The attachment of myristate to the N-terminal glycine of certain proteins is largely a co-translational modification catalyzed by N-myristoyltransferase (NMT), and involved in protein membrane-localization. Using coenzyme A (CoA)-activated lipid, NMT transfers myristate to the substrate protein, after removal of the initiator methionine, in a predominantly co-translational process (Ritzefeld et al., 2017, Schlott et al., 2018). Pathogen NMT is a validated therapeutic target in numerous infectious diseases including malaria. PvNMT possesses 80% sequence identity and 93% similarity to PfNMT and is an excellent platform for structural studies, while to date PfNMT has proven intractable for X-ray crystallography.

IMP-1002 is a previously undisclosed member of our recently reported series of human NMT inhibitors (Mousnier et al., 2018), and a close analog of IMP-0917 that was discovered through a fragment reconstruction approach based on hits from screens against PvNMT and PfNMT. With parasite growth half maximal effective concentration (EC50) inhibitory activity of 34 nM, IMP-1002 is 4-fold more potent in killing parasites than the most potent previously reported PfNMT inhibitor DDD85646 (Wright et al., 2014). For PvNMT[WT] with bound IMP-1002, Y211 adopts rotamer Y211c, allowing the π-π stacking interaction with IMP-1002, which likely results in the increased potency and selectivity (over HsNMT) of this compound compared with DDD85646. Consistent with the high affinity of IMP-1002 for the PvNMT[WT] this protein was stabilized by >8.8°C with 5 μM of IMP-1002 even in the absence of MyrCoA. IMP-1002 and IMP-0917 exhibited interesting kinetics: both showed a slow dissociation rate with PvNMT[WT], suggesting that several hours may be required for complete dissociation. Data from the PfNMT[G386E]-resistant parasite line were used to guide biochemical and structural analysis of this variant in recombinant PvNMT, providing both enzymatic inhibition data and the crystal structures of the WT and G386E variant with bound MyrCoA and the NMT inhibitor (NMTi) used for mutation selection.

>[3x]MGSSHHHHHHSAALEVLFQGPDYKFWYTQPVPKINDEFNESVNEPFISDNKVEDVRKDEYKLPPGYSWYVCDVKDEKDRSEIYTLLTDNYVEDDDNIFRFNYSAEFLLWALTSPNYLKTWHIGVKYDASNKLIGFISAIPTDICIHKRTIKMAEVNFLCVHKTLRSKRLAPVLIKEITRRINLENIWQAIYTAGVYLPKPVSDARYYHRSINVKKLIEIGFSSLNSRLTMSRAIKLYRVEDTLNIKNMRLMKKKDVEGVHKLLGSYLEQFNLYAVFTKEEIAHWFLPIENVIYTYVNEENGKIKDMISFYSLPSQILGNDKYSTLNAAYSFYNVTTTATFKQLMQDAILLAKRNNFDVFNALEVMQNKSVFEDLKFGEGDGSLKYYLYNWKCASFAPAHVGIVLL> ATTPTMQSTSLLTEHLGYPPISLVDDIINAVNEIMYKCTNAMEKYLMQRNIIGKKDFSDEIKIGTAKLESLLENSVDKNFDKLELYVLRNILSIPSDLLEENRFRLLHHEKLVLTDSATR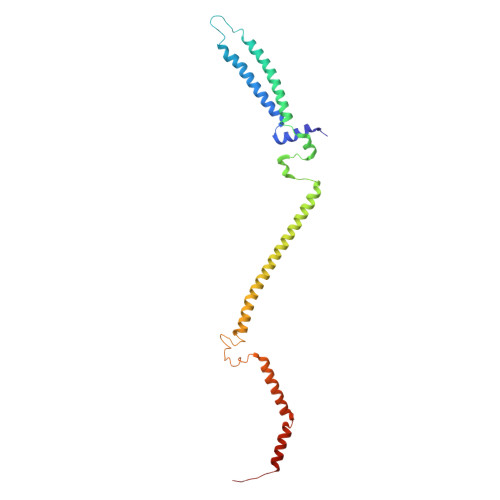AHTDTSIEQKLQEIERQYQLNVMLRDRIQNTKELLTEVVQFKKKVIDLLRCDDNLTTALHELWDDLKPLDVAVKLITTRLKQIYLENEEFYSIDQVNRLVKRYNELRNTSIVR> MSQPQSSQVTKRGLTDPERAAIIAAAVPDHALDTQRKYHYFIQPRWKPLSEYEQLSCYAQPNPDWIAGGLDWGDWTQKFHGGRPSWGNESTELRTTDWYRHRDPARRWHHPYVKDKSEEARYTQRFLAAYSSEGSIRTIDPYWRDE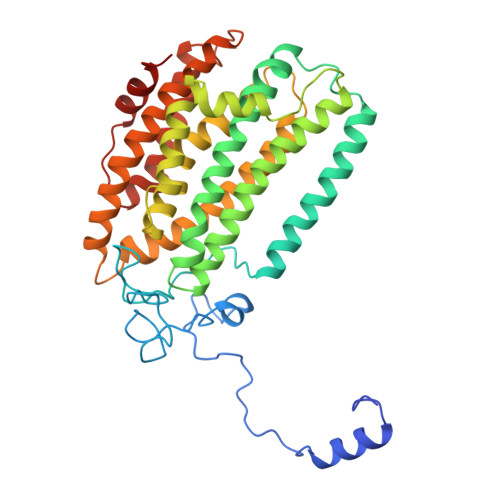ILNKYFGALLYSEYGLFNAHSSVGRDCLSDTIRQTAVFAALDKVDNAQMIQMERLFIAKLVPGFDASTDVPKKIWTTDPIYSGARATVQEIWQGVQDWNEILWAGHAVYDATFGQFARREFFQRLATVYGDTLTPFFTAQSQTYFQTTRGAIDDLFVYCLANDSEFGAHNRTFLNAWTEHYLASSVAALKDFVGLYAKVEKVAGATDSAGVSEALQRVFGDWKIDYADKIGFRVDVDQKVDAVLAGYKN>MDHSITASYYDTTQQLSLLKHVLSEDKRPIAFIIAAGCPVSIRHNDAPLIPDVAGLTRKISDSFGGNPDSLLMKIIQNLKTTIPNPTIEDILSYIRLLQQIPMSGKIHDVENSVINALEESICELIEEEVNVDLPGNATPYHKIAAWINSINREHQVEIFTTNYDLLMEQALEELNVPYFDGFVGSKRAFFDIRTIEENKLPSRWSKLWKLHGSINWQLDKQTQTIWRGTPSKGCSLIHPSHLKYDQSRKMPYLVMMDQLKLFLNQP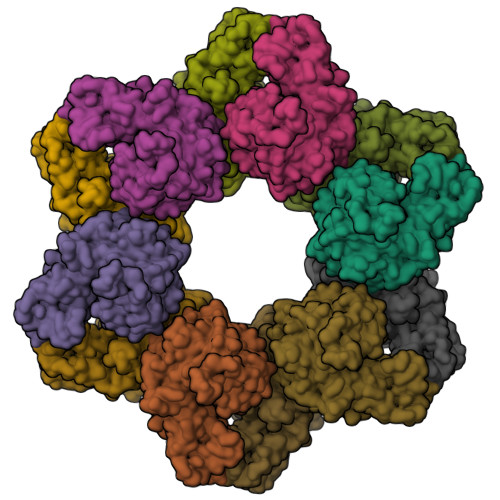SAILITCGYSYKDQHINEVLSQGLQTNPNALIYGLQYDVLENYQEAKDMALKRSNLILLAKDRAIIGKKEGEWKPDPQSSQDNDPLLFFKLGDFQHLASFLEEISQYDWSKQND[12x]>MDKPLKLYFIPYLAAGHMIPLCDIAALFASRGHFVTIITTPLNAKILPKYNNFNVHTFQFPSQEVGLPEGVENLSAVTDLDGAYKIYQAMALLREHIENFVEQHPPDCIVADFLLPWVDELANKLSIPRLAFNGFSLFTICAMESLRSHPLPEDASGPFVIPNFPQDIVINSTPPAESKTFMDPLFTIALKSNGFIINSFVEFDGEEYVKYYEKTIGHKAWHLGPASLVRETIQEKAERGEKSTLSVQKFVDWLNKKRDNSVIYISFGTMCHFPDKQLFEIASAIEASGYDFIWVVPEKKGKENESEDDKEKWLPKGF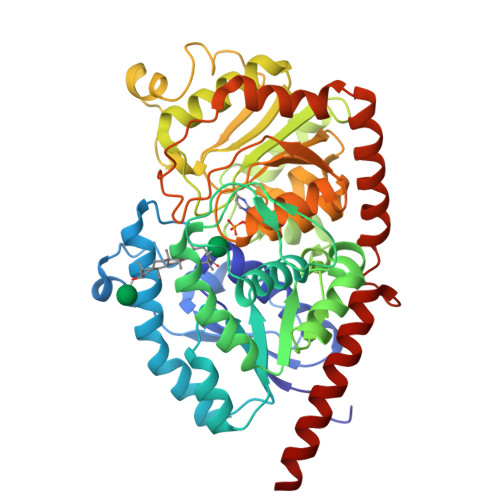EERDNGMIVKGWSPQMVILGHPAVGAFLTHCGWNSTVEAVSAGVPMITWPVLGDQFYNEKLITQVRGIGVEVGVDEWVVTSFRGMKQLVGRDCIEKAIRRLMDGGDEAIQIRERSQKLAKITKHVVQEGGSSYENLTVLINELKQLRDCKVLN[4x]>NRWGLIGASTIAREWVIGAIRATGGEVVSMMSTSAERGAAYATENGIGKSVTSVEELVGDPDVDAVYVSTTNELHRE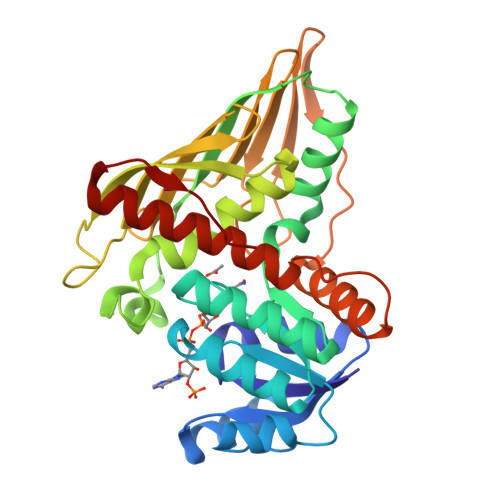QTLAAIRAGKHVLCEKPLAMTLEDAREMVVAAREAGVVLGTNHHLRNAAAHRAMRDAIAEGRIGRPIAARVFHAVYLPPHLQGWRLERPEAGGGVILDITVHDADTLRFVLNDDPAEAVAISHSAGMGKEGVEDGVMGVLRFQSGVIAQFHDAFTTKFAETGFEVHGTEGSLIGRNVMTQKPVGTVTLRNAEGESQLPLDPANLYETALAAFHSAIEGHGQPSATGEDGVWSLATGLAVVKAAATGQAAEIETGL[6x]> MQRIIVNPNEPYLSVIKKVVKLSIPIIVVNLLYTVENMISMILVSSISPSAVAATGFSLSLLWFIYSLMALSYSGTNILIAQFVGAKKDPSPILINGLFLSFLISLPLFFYGKDFVLFLMKVLGASETVRSLAKEYLTPIFWFIPIGFLTNTFYGAYNGAGD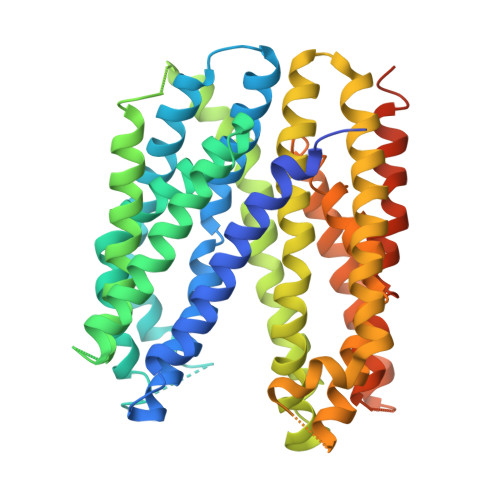TKTPMKVAIIMNLTHIGTAYTLINGKFGLPKLGVEGAGWGIAISEILAFFIYTFLLIFFKKPFPLHLRLEPKLLFKMVRLGTPTALERAITTLSFNVFVGFLAKFGDKVLAAHQIGLRIESISFMIGFGVMIASTTLAGQNYGARNYRGMVHAVNTSAHFTALVMSLTGLILILFPHYLVYPFSRDPEVIEWASYYLQIVGISQPAMAYASIYSGALKGMGKTHIPLFVNISSFWLFRIIPSYFLLKVIHSPLVPWGFMTFETAVRALFYYTVFKKVVGKLLQTFQKEEEPEGEDAEGDKPLDEVRSKVT>[4x]SMMIEFLNLRGKRALITAGTKGAGAATVSLFLELGAQVLTTARARPEGLPEELFVEADLTTKEGCAIVAEATRQRLGGVDVIVHMLGGSSAAGGGFSALSDDDWYNELSLNLFAAVRLDRQLVPDMVARGSGVVVHVTSIQRVLPLPESTTAYAAAKAALSTYSKAMSKEVSPKGVRVVRVSPGWIETEASVRLAERLAKQAGTDLEGGKKIIMDGLGGIPLGRPAKPEEVAN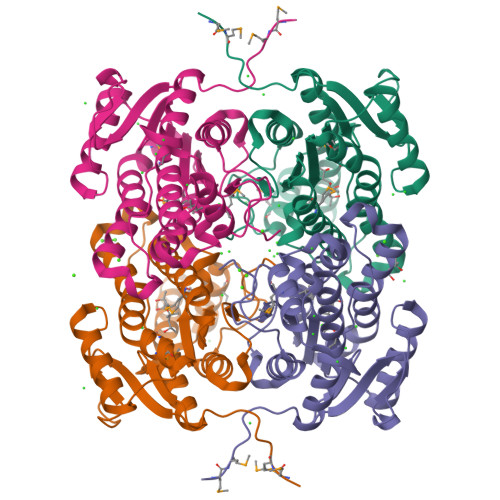LIAFLASDRAASITGAEYTIDGGTVPTA(1R,3R)-5-[(2E)-2-[(1R,3aS,7aR)-1-[(2R,3S)-3-(2-hydroxyethyl)nonan-2-yl]-7a-methyl-2,3,3a,5,6,7-hexahydro-1H-inden-4-ylidene]ethylidene]-2-methylidene-cyclohexane-1,3-diol 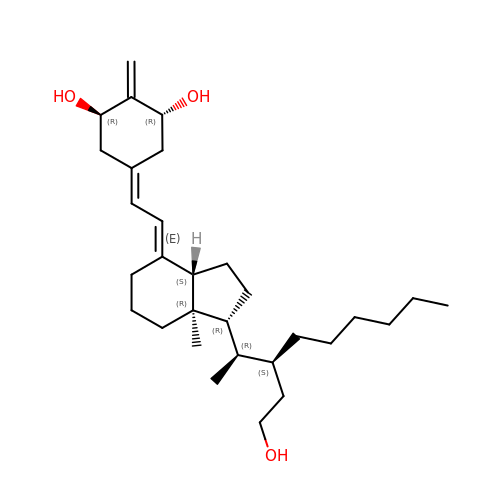| C30 H50 O3 | JUQILRKVRIIJNO-FJOOTJEJSA-N>[2x]MQFFGRLVNTLSSVTNLFSNPFRVKEISVADYTSHERVREEGQLILFQNASNRTWDCILVSPRNPHSGFRLFQLESEADALVNFQQFSSQLPPFYESSVQVLHVEVLQHLSDLIRSHPSWTVTHLAVELGIRECFHHSRIISCANSTENEEGCTPLHLACRKGDSEILVELVQYCHAQMDVTDNKGETAFHYAVQGDNSQVLQLLGKNASAGLNQVNKQGLTPLHLACQMGKQEMVRVLLLCNARCNVMGPSGFPIHTAMKFSQKGCAEMIISMDSSQIHSKDPRYGASPLHWAKNAEMARMLLKRGCDVDSTSAAGNTALHVAVMRNRFDCVMVLLTYGANAGTPGEHGNTPLHLAISKDNMEMIKALIVFGAEVDTPNDFGETPAFMASKISKQLQDLMPISRARKPAFILSSMRDEKRIHDHLLCLDGGGVKGLVIIQLLIAIEKASGVATKDLFDWVAGTSTGGILALAILHSKS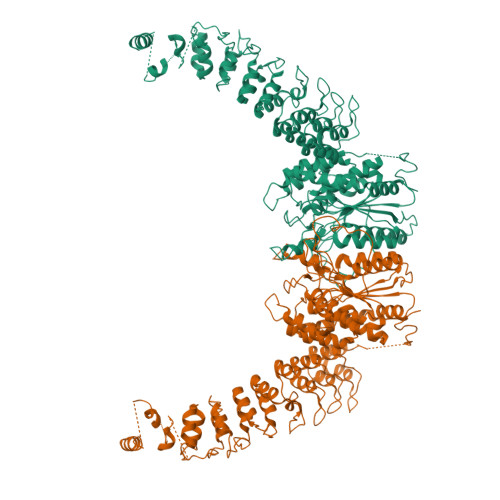MAYMRGVYFRMKDEVFRGSRPYESGPLEEFLKREFGEHTKMTDVKKPKVMLTGTLSDRQPAELHLFRNYDAPEVIREPRFNQNINLKPPTQPADQLVWRAARSSGAAPTYFRPNGRFLDGGLLANNPTLDAMTEIHEYNQDMIRKGQGNKVKKLSIVVSLGTGRSPQVPVTCVDVFRPSNPWELAKTVFGAKELGKMVVDCCTDPDGRAVDRARAWSEMVGIQYFRLNPQLGSDIMLDEVNDAVLVNALWETEVYIYEHREEFQKLVQMLLSP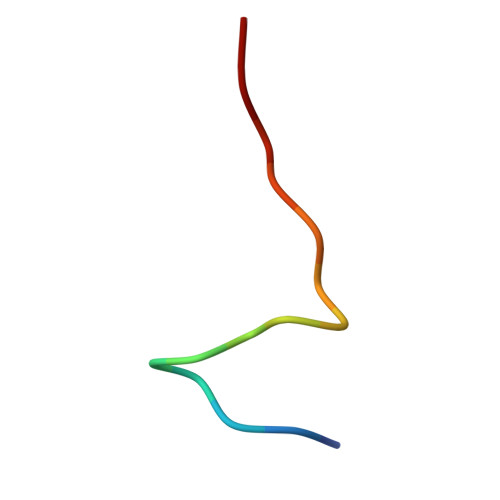> AAAAAAETDWKVIAA FtsEX is a transmembrane signaling complex that coordinates periplasmic peptidoglycan remodelling with cytoplasmic cell division events. pneumoniae, FtsEX interacts directly with peptidoglycan hydrolases such as PcsB, but in Escherichia coli, and other gram-negative bacteria, FtsEX interacts with a periplasmic intermediary, EnvC, that activates downstream amidases. EnvC is termed a “murein hydrolase activator” and has been shown to stimulate peptidoglycan hydrolysis by both AmiA and AmiB in vitro. FtsEX functions in bacterial cell division and regulates periplasmic amidases such as AmiA and AmiB via its interaction with the murein hydrolase activator, EnvC.

Here we present a 2.1 Å crystal structure of EnvC bound to the periplasmic domains of FtsX, revealing the molecular underpinnings of this interaction and the first complete structure of EnvC. Crystals of the EnvC-FtsX periplasmic domain complex belong to space group P212121 with two molecules of the FtsX periplasmic domain and one molecule of EnvC in the asymmetric unit. A groove in the surface of the LytM domain forms the amidase recruitment site which is here found to be blocked by the regulatory domain. Occupation of the amidase-binding site by the restraining arm strongly suggests that EnvC has been captured in an autoinhibited state that would necessitate a conformational change in order to bind and activate its cognate amidases. The N-terminal coiled coil domain of EnvC has a hairpin-like structure formed by a pair of antiparallel coiled coil helices (long helices I and II) that are joined by a short linker. The two interfaces are mostly hydrophobic and dominated by interactions arising from the X-lobe (residues 145 to 171) which partially wraps around each of the two long helices that make up the EnvC coiled coil. Phe158 is notable for its position at the tip of the X-lobe where it slots between the two antiparallel helices of EnvC, locking each FtsX domain in place. The set of FtsX residues contacting the two EnvC-binding sites are nearly identical for both interfaces, suggesting the same molecular surface recognizes two structurally distinct target sites—an example of dual recognition. As shown here, the FtsEX-EnvC interaction involves a single EnvC monomer locked between the two periplasmic domains via interactions with both the X-lobe and the Porter domain (2:1).

> MDERDQLKSIQADIAAKERAVRQKQQQRASLLAQLKKQEEAISEATRKLRETQNTLNQLNKQIDEMNASIAKLEQQKAAQERSLAAQLDAAFRQGEHTGIQLILSGEESQRGQRLQAYFGYLNQARQETIAQLKQTREEVAMQRAELEEKQSEQQTLLYEQRAQQAKLTQALNERKKTLAGLESSIQQGQQQLSELRANESRLRNSIARAEAAAKARAEREAREAQAVRDRQKEATRKGTTYKPTESEKSLMSRTGGLGAPRGQAFWPVRGPTLHRYGEQLQGELRWKGMVIGASEGTEVKAIADGRVILADWLQGYGLVVVVEHGKGDMSLYGYNQSALVSVGSQVRAGQPIALVGSSGGQGRPSLYFEIRRQGQAVNPQPWLGR;>[2x]MGQITVYLQKTLDDDAAAGVVAQLQAEQGVEKVNYLSREDALGEFRNWSGFGGALDMLEENPLPAVAVVIPKLDFQGTESLNTLRDRITQINGIDEVRMDDSLEHHHHHH> 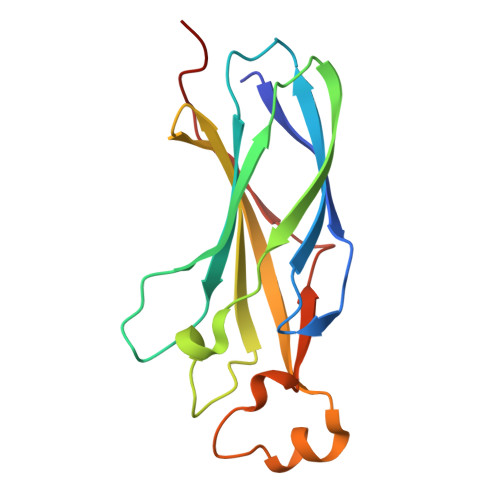GAMSIVSLLGIKVLNNPAKFTDPYEFEITFECLESLKHDLEWKLTYVGSSRSLDHDQELDSILVGPVPVGVNKFVFSADPPSAELIPASELVSVTVILLSCSYDGREFVRVGYYVNNEYDEEELRENPPAKVQVDHIVRNILAEKPRVTRFNIVWDNE>[9x]MQRLFLLVAVMLLSGCLTAPPKEAARPTLMPRAQSYKDLTHLPAPTGKIFVSVYNIQDETGQFKPYPASNFSTAVPQSATAMLVTALKDSRWFIPLERQGLQNLLNERKIIRAAQENGTVAINNRIPLQSLTAANIMVEGSIIGYESNVKSGGVGARYFGIGADTQYQLDQIAVNLRVVNVSTGEILSSVNTSKTILSYEVQAGVFRFIDYQRLLEGEVGYTSN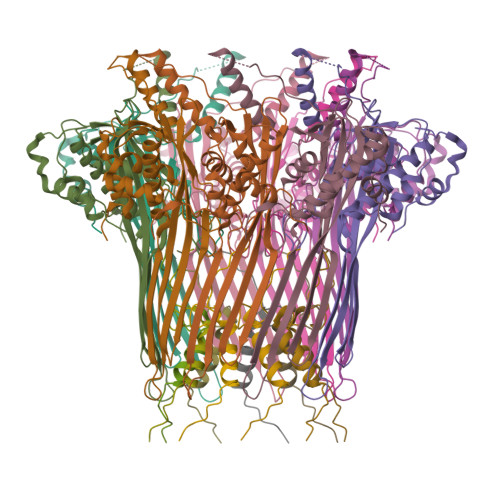EPVMLCLMSAIETGVIFLINDGIDRGLWDLQNKAERQNDILVKYRHMSVPPES;>MRVKHAVVLLMLISPLSWAGTMTFQFRNPNFGGNPNNGAFLLNSAQAQNSYKDPSYNDDFGIETPSALDNFTQAIQSQILGGLLSNINTGKPGRMVTNDYIVDIANRDGQLQLNVTDRKTGQTSTIQVSGLQNNSTDF[9x]> DYAPTKLLPQQ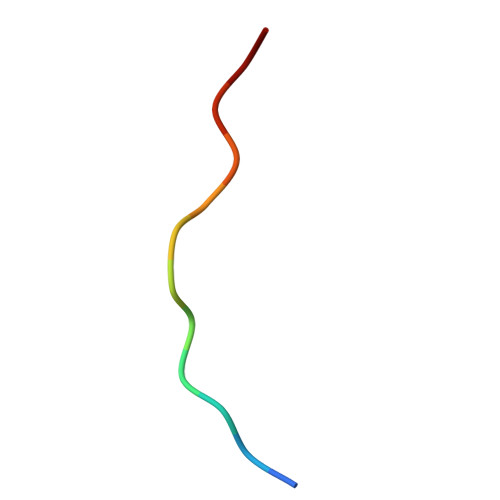P>MSSNPHRWMMTSPGAPMVRAEFEIGELSADQVVVAVAGCGVCHTDLGYYYDSVRTNHALPLALGHEISGRVVQAGANAAQWLGRAVIVPAVMPCGTCELCTSGHGTICRDQVMPGNDIQGGFASHVVVPARGLCPVDEARLAAAGLQLADVSVVADAVTTPYQAVLQAGVEPGDVAVVIGVGGVGGYAVQIANAFGASVVAIDVDPAKLEMMSKHGAALTLNAREISGRDLKKAIEAHAKANGLRLTRWKIFECSGTGAGQTSAYGLLTHGATLAVVGFTM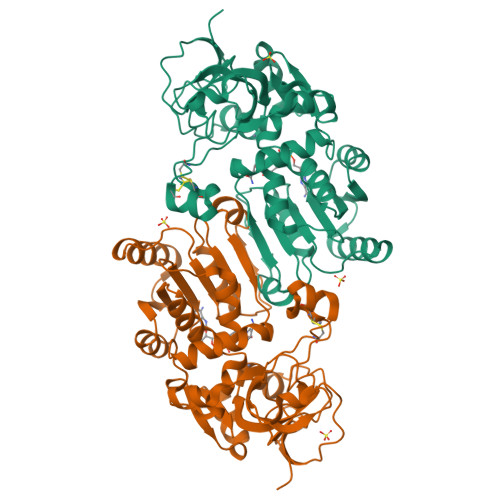DKVEVRLSNLMAFHARALGNWGCLPEYYPAALDLVLDKKIDLASFIERHPLDQIGEVFAAAHAHKLTRRAILT[3x]> MEKSVSVILLAGGQGKRMKMSMPKQYIPLLGQPIALYSFFT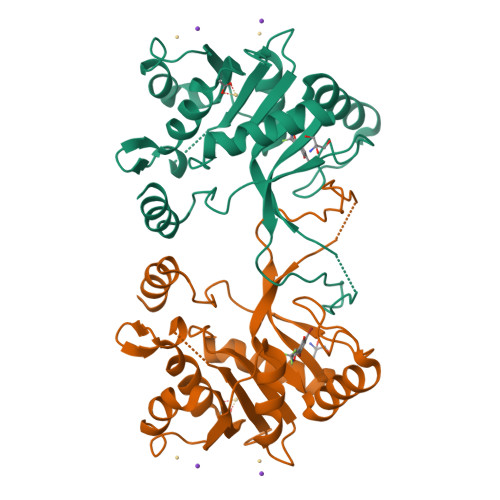FSRMPEVKEIVVVCDPFFRDIFEEYEESIDVDLSFAIPGKERQDSVYSGLQEIDVNSELVCIHDSARPLVNTEDVEKVLKDGSAVGAAVLGVPAKATIKEVNSDSLVVKTLDRKTLWEMQTPQVIKPELLKKGFELVKSEGLEVTDDVSIVEYLKHPVYVSQGSYTNIKVTTPDDLLLAERILSEDS> MKEFYLTVEQIGDSIFERYIDSNGRERTREVEYKPSLFAHCPESQATKYFDIYGKPCTRKLFANMRDASQWIKRMEDIGLEALGMDDFKLAYLSDTYNYEIKYDHTKIRVANFDIEVTSPDGFPEPSQAKHPIDAITHYDSIDDRFYVFDLLNSPYGNVEEWSIEIAAKLQEQGGDEVPSEIIDKIIYMPFDNEKELLMEYLNFWQQKTPVILTGWNVESFAIPYVYNRIKNIFGESTAKRLSPHRKTRVKVIENMYGSREIITLFGISVLDYIDLYKKFSFTNQPSYSLDYISEFELNVGKLKYDGPISKLRESNHQRYISYNIIAVYRVLQIDAKRQFINLSLDMGYYAKIQIQSVFSPIKTWDAIIFNSLKEQNKVIPQGRSHPVQPYPGAFVKEPIPNRYKYVMSFDLTSMYPSIIRQVNISPETIAGTFKVAPLHDYINAVAERPSDVYSCSPNGMMYYKDRDGVVPTEITKVFNQRKEHKGYMLAAQRNGEIIKEALHNPNLSVDEPLDVDYRFDFSDEIKEKIKKLSAKSLNEMLFRAQRTEVAGMTAQINRKLLINSLYGALGNVWFRYYDLRNATAITTFGQMALQWIERKVNEYLNEVCGTEGEAFVLYGDTDSIYVSADKIIDKVGESKFRDTNHWVDFLDKFARERMEPAIDRGFREMCEYMNNKQHLMFMDREAIAGPPLGSKGIGGFWTGKKRYALNVWDMEGTRYAEPKLKIMGLETQKSSTPKAVQKALKECIRRMLQEGEESLQEYFKEFEKEFRQLNYISIASVSSANNIAKYDVGGFPGPKCPFHIRGILTYNRAIKGNIDAPQVVEGEKVYVLPLREGNPFGDKCIAWPSGTEITDLIKDDVLHWMDYTVLLEKTFIKPLEGFTSAAKLDYEKKASLFDMF

The replicative DNA pol from bacteriophage RB69 (RB69pol) is a member of the B family and is responsible for DNA synthesis of both leading and lagging strands of its genome. It has extensive sequence similarity to human replicative pols α and δ and therefore has been regarded as a good model for B family pols. Our previous reported 1.8 Å resolution structure of wt RB69pol showed that L415 is located right below the triphosphate tail of the incoming dNTP, where a small hydrophobic cavity exists at the tip of the L415 side chain. To provide a structural basis that could account for the different kinetic behavior observed among L415 variants and wt RB69pol, we determined the crystal structures of three ternary complexes: dTTP/dA-with the L415A mutant; dATP/dT-with the L415G mutant and dATP/dT-with the L415M mutant with resolutions ranging from 1.80 to 2.04 Å and Rfree values ranging from 21.3% to 21.9%.

In contrast to the L415A and L415G mutants, the L415 to Met substitution did not disturb the adjacent residues. The side chain of M415 is snuggly accommodated in the pocket surrounded by Y416, G590 and L412, thus fully occupying the cavity present in wt RB69pol. Interestingly, the rotameric position of D411 as observed in the wt structure is restored in the L415M mutant. Overall, the structure of the L415M ternary complex is much closer to the structure of the wt RB69pol ternary complex than the structure of either the L415A or L415G ternary complexes. Accommodation of the M415 side chain in the hydrophobic cavity without disturbing the nearby residues could provide an energetic advantage to this mutant over wt RB69pol forming the conformation required for dNTP incorporation. A more rigid anchor of the metal ions would likely facilitate the alignment between the 3′-OH and Pα of the incoming dNTP. Together, these structural interpretations help explain the increased catalytic efficiency of the L415M mutant over wt RB69pol. Interestingly, when L415 was replaced with Met, an amino acid with a longer side-chain, the base selectivity was not compromised. In contrast, the L415 to Met substitution would be expected to restrict the movement of nearby residues. Therefore, the partitioning between the pol and exo domains is not significantly compromised with the L415M mutant.In humans, the CALHM family encompasses six paralogs, some of which function as non-selective channels that are permeable to large substances such as ATP. We identified the three paralogs, CALHM2, 4 and 6, to be highly expressed in this organ. The CALHM subunits thus constitute unique modular building blocks that assemble with different stoichiometries into large membrane channels. In contrast to previously described CALHM structures, where the oligomeric state of individual channels was described as uniform, our data show heterogeneous populations with CALHM4 and CALHM6 assembling as decameric and undecameric channels with similar abundance and CALHM2 as predominantly undecameric proteins with a smaller population of dodecamers (Figure 3—figure supplements 2–4 and 6). Despite the unknown activating stimuli, our study has provided insight into gating transitions of CALHM channels by showing two conformations with either a cylindrical pore of uniform large dimeter within the membrane that is constricted at the intracellular side as in case of CALHM4 and a conical pore that continuously narrows from its extracellular entry towards the cytoplasm as in case of CALHM6.

In each case, we found a heterogeneous, about equal distribution of particles with two distinct oligomeric states. The smaller particles are composed of decameric and the larger of undecameric assemblies, both of which we refer to as CALHM4 channels. Due to the slightly higher quality of the Ca2+-free sample, we continued to use this data for our further analysis unless specifically indicated. The cryo-EM density of the decamers extends to a resolution of 4.1 Å and undecamers to 3.7 Å, which in both cases permitted the unambiguous interpretation by an atomic model (Figure 3—figure supplements 2, 3 and 5A). In each structure, the subunits are arranged around a central axis of symmetry that defines the ion-conduction path. Both assemblies contain pairs of CALHM4 channels of the same size related by two-fold symmetry that interact via their cytoplasmic parts. In the plane of the membrane, the dimensions of decameric and undecameric CALHM4 channels amount to 110 Å and 120 Å respectively. The diameter at both entrances of the pore measures about 52 Å and 60 Å for decameric and undecameric assemblies respectively, thus defining the properties of an unusually large channel, which could be permeable to molecular substrates. Even at the constriction located at the intracellular membrane leaflet where the respective N-terminal helices NH project towards the pore axis, the decameric channels are about 20 Å and undecameric channels 30 Å wide. In both cases the pore would thus be sufficiently large to accommodate an ATP molecule, consistent with the notion of CALHM proteins forming ATP-permeable channels.

>MCPTLNNIVSSLQRNGIFINSLIAALTIGGQQLFSSSTFSCPCQVGKNFYYGSAFLVIPALILLVAGFALRSQMWTITGEYCCSCAPPYRRISPLECKLACLRFFSITGRAVIAPLTWLAVTLLTGTYYECAASEFASVDHYPMFDNVSASKREEILAGFPCCRSAPSDVILVRDEIALLHRYQSQMLGWILITLATIAALVSCCVAKCCSPLTSLQHCYWTSHLQNERELFEQAAEQHSRLLMMHRIKKLFGFIPGSEDVKHIRIPSCQDWKDISVPTLLCMGDDLQGHYSFLGNRVDEDNEEDRSRGIELKP[20x]> MRGSHHHHHHGSALPILLDCDPGHDDAIAIVLALASPELDVKAITSSAGNQTPEKTLRNVLRMLTLLNRTDIPVAGGAVKPLMRELIIADNVHGESGLDGPALPEPTFAPQNCTAVELMAKTLRESAEPVTIVSTGPQTNVALLLNSHPELHSKIARIVIMGGAMGLGNWTPAAEFNIYVDPEAAEIVFQSGIPVVMAGLDVTHKAQIHVEDTERFRAIGNPVSTI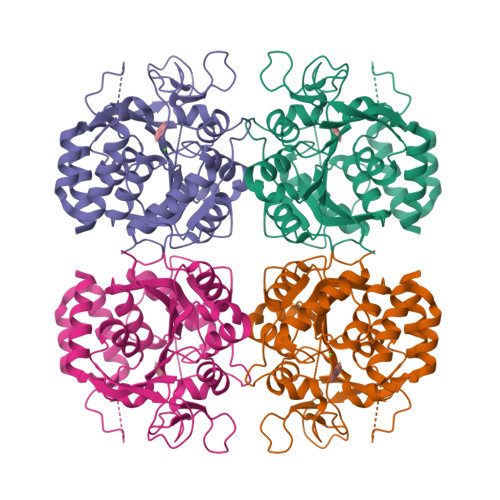VAELLDFFLEYHKDEKWGFVGAPLHDPCTIAWLLKPELFTSVERWVGVETQGKYTQGMTVVDYYYLTGNKPNATVMVDVDRQGFVDLLADRLKFYA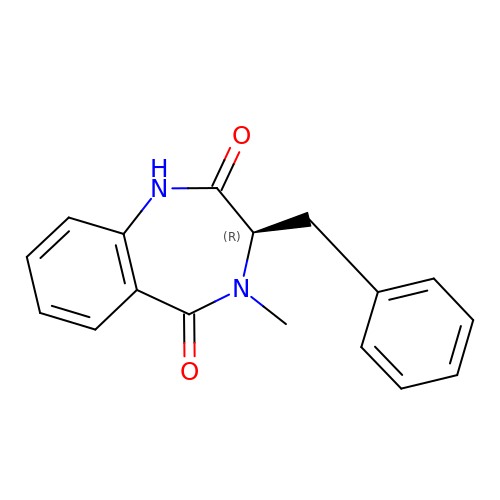(3R)-4-methyl-3-(phenylmethyl)-1,3-dihydro-1,4-benzodiazepine-2,5-dione | C17 H16 N2 O2 | KSQNKZMAMGACTL-OAHLLOKOSA-N>[6x]M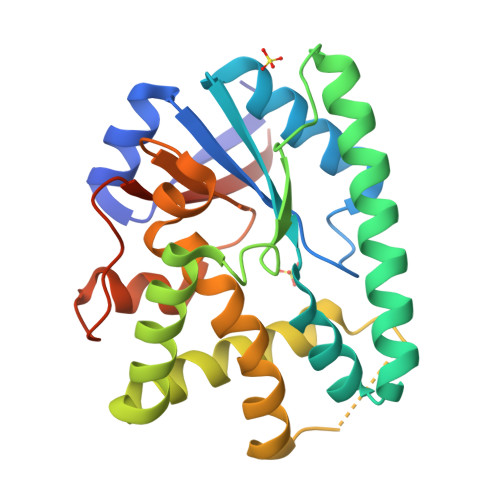QNFKVDFLTKNCKQIYQRKKHVILGISPFTSKYNESYIRKIIQWANSNFDDFSILLAGEESKNLLECLGYSSSKANQKVRKEIKRQIRFCEDEIIKCNKTITNRIHRFSDFKNNIYYIDIYKTIVDQFNTDSNFKNSCLKMSLQALQSKGKNVNTSIEITDETLEYAAQYVLAELPFFLNANPIINTQETLMAYHAPWELGTNIINDQFNLKMNEKQGYIILTEKGDNYVKSV> MTYGPILKQLLSPYFSGRVFPDAAPDVPGQDPYVIYQRVGGIPTYFTEGALADKANARVQLEVWSTSKQATYEAMVHIMRSVAAAPAMEPLGQPIDDYEPALRIYGSRV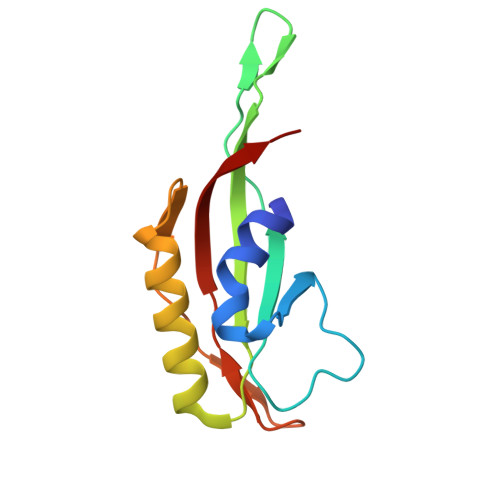DISMYYNLT>MKKGHHHHHHGSERTGTQPLGVQGLTEEQRMMIRELMDAQMKTFDTTFSHFKNFRLPGVLSSGCELPESLQAPSREEAAKWSQVRKDLCSLKVSLQLRGEDGSVWNYKPPADSGGKEIFSLLPHMADMSTYMFKGIISFAKVISYFRDLPIEDQISLLKGAAFELCQLRFNTVFNAETGTWECGRLSYCLEDTAGGFQQLLLEPMLKFH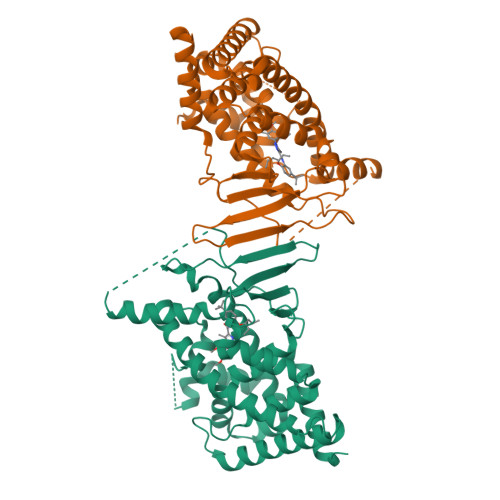YMLKKLQLHEEEYVLMQAISLFSPDRPGVLQHRVVDQLQEQFAITLKSYIECNRPQPAHRFLFLKIMAMLTELRSINAQHTQRWLRIQDIHPFATPLMQELFGITGSSGGSGGSSHSSLTERHKILHRLLQEGSPSDITTLSVEPD[2x]The osmoregulatory ABC transporter OpuA protects Lactococcus lactis against hyperosmotic stress by accumulating the compatible solute glycine betaine. The SBD of OpuA, hereafter named OpuAC, belongs to a superfamily of proteins associated with ABC transporters involved in solute uptake in prokaryotes. The structures of OpuAC showed a fold typical of SBD's, having two α/β domains that enclose a ligand-binding site when in contact with each other. OpuAC is highly specific for glycine betaine and the related proline betaine.

OpuAC was crystallized in the absence and presence of 1 mM glycine betaine, yielding an open conformation (space group P41212, diffracting to 1.9 Å resolution) and closed-liganded conformation (space group H32, diffracting to 2.2 Å resolution), respectively. In the open conformation, the α/β domains had moved by 25° relative to one another when compared to the closed-liganded state. OpuAC belongs to Class II of the proteins in the SBD family, with two connecting segments forming the hinge, of which the central residues are Lys404 and Ser508. In the open conformation structure, electron density was observed in the binding site, although it could not be unambiguously assigned to glycine betaine. Electron density was observed in the ligand-binding site of the open conformation structure. This density could not unambiguously be determined, but likely represents endogenous ligand that was co-purified with the protein, as ITC and fluorescence titration experiments showed that the amount of substrate bound per mol OpuAC was below 1. On the basis of modeling and refinement of the ambiguous density as glycine betaine, the initial coordination of the quaternary ammonium moiety would be performed by W377.

> DKKVDLVYMNWDSEVASINVLTQAMKEHGFDVKTTALDNAVAWQTVANGQADGMVSAWLPNTHKTQWQKYGKSVDLLGPNLKGAKVGFVVPSYMNVNSIEDLTNQANKTITGIEPGAGVMAASEKTLNSYDNLKDWKLVPSSSGAMTVALGEAIKQHKDIVITGWSPHWMFNKYDLKYLADPKGTMGTSENINTIVRKGLKKENPEAYKVLDKFNWTTKDMEAVMLDIQNGKTPEEAAKNWIKDHQKEVDKWFKGS> DTSHHDQDHPTFNKITPNLAEFAFSLYRQLAHQ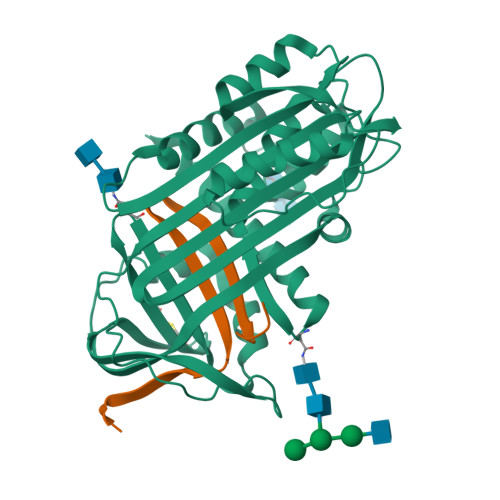SNSTNIFFSPVSIATAFAMLSLGTKADTHDEILEGLNFNLTEIPEAQIHEGFQELLRTLNQPDSQLQLTTGNGLFLSEGLKLVDKFLEDVKKLYHSEAFTVNFGDTEEAKKQINDYVEKGTQGKIVDLVKELDRDTVFALVNYIFFKGKWERPFEVKDTEEEDFHVDQVTTVKVPMMKRLGMFNIQHCKKLSSWVLLMKYLGNATAIFFLPDEGKLQHLENELTHDIITKFLENEDRRSASLHLPKLSITGTYDLKSVLGQLGITKVFSNGADLSGVTEEAPLKLSKAVHKAVLTIDEKGTEAAGAMFLEAIPM;> SIPPEVKFNKPFVFLMIEQNTKSPLFMGKVVNPTQK Nhe is a complex pore-forming toxin (PFT) consisting of three proteins, NheA (41-kDa), NheB (39-kDa), NheC (40-kDa), encoded by one operon containing three genes nheA, nheB and nheC, respectively. Separately, these proteins show no toxicity, but as a binary complex some activities (NheA + NheB: ~5%) were seen and maximal activity is obtained only when all three components are presented (100%). The NheB and NheC components are able to bind to cell membranes, whereas NheA was believed to lack this ability, despite the fact that binding of NheA to NheB/NheC is thought to be the final stage of pore formation. In conclusion, the structure of NheA has revealed an architecture showing it to be, like Hbl-B, a member of the ClyA toxin superfamily of α-pore forming toxins (α-PFTs).

We report here the crystal structure determination at 2.05 Å resolution of NheA by selenomethione Multiwavelength Anomalous Dispersion (MAD). The NheA crystal structure shows that there are eight copies of the NheA molecule in the asymmetric unit. There was no evidence of oligomerization as all eight molecules of NheA all appear to be monomeric using the criteria of PDBePISA. Excluding these regions of disorder, the alpha carbons of the eight molecules superpose on one another with an RMSD of 0.3-0.4 Å and therefore can be considered as almost identical. As expected from the structures of Hbl-B and ClyA, with which NheA has 20% and 18% sequence identity respectively, the structure of NheA is predominantly composed of α-helices with approximate dimensions of 95Å x 40Å x 20Å. The tail domain forms the main body of the structure and consists of five major helices designated: αA (Ser 24- Gln 44); αB (Leu 56 – Gly 104) with a distinct kink at residues TYR 95 and TYR 96; αC (Glu 110 - Leu 166) with a kink at residue Leu 141; αF (Ala 271- Glu 319); and αG (Ser 326 – Thr 355). The head domain includes two long α-helices: αD (Asp 172-Leu 195) and αE (Ser 243-Thr 269) separated by a β-hairpin consisting of two long β strands: strand 1 (Gly 204- Thr 216) and strand 2 (Thr 222- Leu 233). Unlike ClyA the two strands in this hairpin actually form part of a three-stranded β-sheet as Strand 1 forms hydrogen bonds to a third, very short β-strand from the tail domain, which is formed from 4 residues (Val 357, Glu 358, Val 359, His 360) at the C-terminal of the protein. The structure reveals a similar overall fold to B. cereus Hbl-B and E. coli ClyA, but, unlike them, its enlarged "head" domain displays on its surface an enlarged β-tongue which is of amphipathic rather than hydrophobic nature. Intriguingly, we show here that in NheA a β-hairpin of similar sequence appears to be held in position by five hydrogen bonds from a short third β-strand that forms the C-terminal of NheA (red).

>KEGQTEVKTVYAQNVIAPNTLSNSIRMLGSQSPLIQAYGLVILQQPDIKVNAMSSLTNHQKFAKANVREWIDEYNPKLIDLNQEMMRYSIRFNSYYSKLYELAGNINEDEQSKADFTNAYGKLQLQVQSIQENMEQDLLELNRFKTVLDKDSNNLSIKADEAIKTLQGSSGDIVKLREDIKRIQGEIQAELTTILNRPQEIIKGSINIGKQVFTITNQTAQTKTIDFVSIGTLSNEIVNAADSQTREAALRIQQKQKELLPLIQKLSQTEAEATQITFVEDQVSSFTELIDRQITTLETLLTDWKVLNNNMIQIQKNVEEGTYTDSSLLQKHFNQIKKVSDEMNKQTNQFEDYVTNVEVH[8x]(3R)-1-methylpyrrolidin-3-ol | C5 H11 N O | 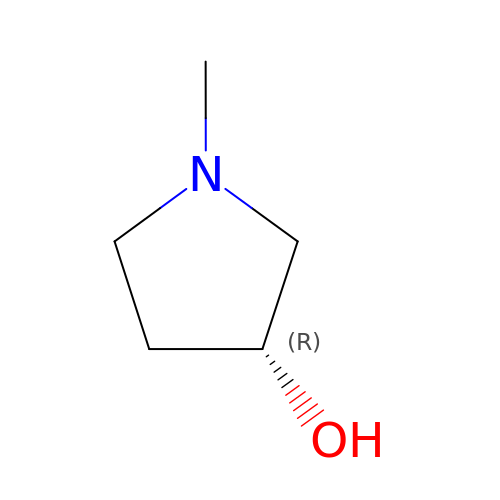FLVFPAIGVBQGET-RXMQYKEDSA-N> TGFDFNAYMGEKAAAVNRALDASIPADEPPAALHEAMRYALLAGGKRVRPALCLAACAVVGGREAWAMPAAAAVEMVHTMSLVHDDLPCMDDDDLRRGKPTCHVVYGEPIAVLTGDALLSLSFHHMARFDSYPPDIDADKHPARVVRAIGELARCIGSEGLVAGQVVDLEMTGSTETVPLERLEYIHLHKTAALLEASVVIGAILGGGSDEQIESLRMYARSIGLLFQVVDDILDVTKSSEELGKTAGKDLA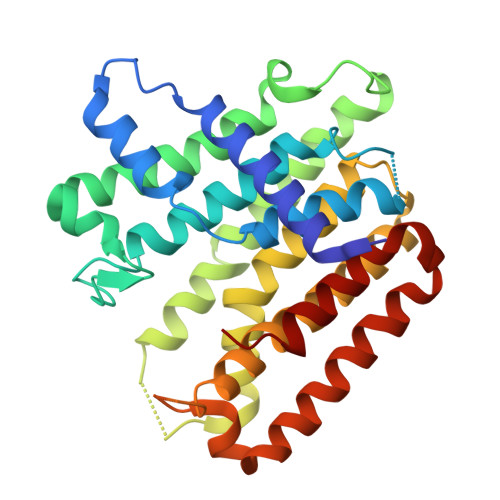SDKTTYPKLLGLEKSREFAEKLLSDAREQLSGFDQETAAPLLHLANYIAYRQN Here we describe a data-driven process for the high-speed, automated creation of stable protein designs. We describe a computationally efficient neural network, the Evaluator Model (EM), that is able to predict protein stability with high accuracy, based solely on amino acid sequence. We describe another neural network, the Generator Model (GM), that is able to create novel stable protein sequences at high speed; these sequences can also be successfully refined by the EM. Finally, we demonstrate via low-resolution methods that selected examples fold into stable structures, and report a high resolution crystal structure of one design that matches the expected topology.

The design began with a requested secondary structure fed into the GM. The GM produced a primary sequence (nmt_0994) stochastically translated from that secondary structure; however, the Reverse GM correctly predicted that two of the requested helices were actually merged into one in the generated protein’s structure. EM-guided refinement then changed two residues to tryptophan, which raised the empirical stability score from -0.18 to 1.88. The nmt_0457_guided_03 and nmt_0994_guided_02 proteins, expected to be all alpha helical, show distinct minima at 222nm and 208nm, consistent with the intended helical structure. Five of the eight monomeric/oligomeric designs are highly thermostable; four do not unfold even at a temperature of 99°C. These four are precisely the non-aggregating proteins with stability score > 1, providing additional experimental validation to the previously published finding that stability scores are reasonably correlated with thermal stability. For one of these highly stable designs we obtained a crystal structure; this showed an all-helical structure, consistent with predictions of the Reverse GM, CD, and AlphaFold2. Two of the three helical segments observed in the crystal structure match AlphaFold2’s prediction, with the third helix taking a slightly different trajectory from the prediction. (C) Crystal structure for nmt_0994_guided_02 (dark grey), showing that it also has the three helices predicted by the Reverse GM for its pre-refinement progenitor. The prediction and the crystal structure have a CαRMSD of 3.4 Å. We found that one such model (trRosetta) could predict the crystal structure that we obtained for one of our designs with reasonable accuracy (CαRMSD of 3.7 Å), including correctly predicting the secondary structure and the relative orientation of secondary-structure elements, despite differences in finer details.

> DEREIARKVASELQKFSEWVKKLKEVIKKASPEQQTKIAQWVAKLAGVRPEDVKKIIKAFND6-(1,1-dioxidothiomorpholin-4-yl)-N-(3-methoxyphenyl)-1-methyl-1H-pyrazolo[3,4-d]pyrimidin-4-amine 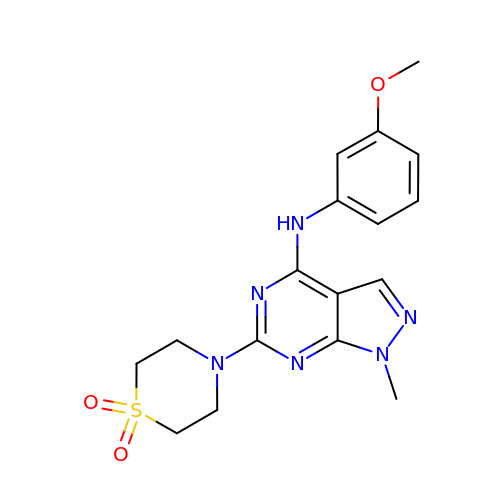| C17 H20 N6 O3 S | IDYJWHSIWMIDKD-UHFFFAOYSA-N> MGSSHHHHHHSQDPENLYFQSMIPQFVIPLTNCLGQSYHFSSQPIPKGEHKKFDSEQSAKAFLDDFVPLRSSRVEELYHLLGQFPPNVPDEELTPELYAPVFAKALVNGSLYVASFPKTKKNATISSEPTPVPKQVKAKSKQNKAHTSSKTQAKNSASAKPLQTGSECHEKAGDPVSLVTGAEILTLNDVELPNGFVWSRTYRSSKASRNQGLGYGWRHAFQFELKEVTDEKHNVTSWEFISDSADEIEFEPVEHGSTSYQVYVGASCHFLNPNIRIVTLSSGDQYRFELVEDIWLLKQVRNGIFSTFQLRYSRNHRLIEVAHNKRPVLECQYDKQGRLVELLNAKTEQVLTTYIYDEQDDLVGATNDLGLTERYEYQDQHLIAKRVRPTGFTHYFEWSGEGSSAKCIRNFGDSGIYDYRFHYEGAKSSYSDSLDNEWTFIHDEQGHLLEKSSPTGRTWQWHYDHLGRKEKAVFPDNSTTQYQYNQQGQLISKLHSSGAQIQYGYDSLGKLVKTVSPDGDLEKAYYNSLGQRVWDIDALGCVTEYEYDKHGQVVKRESEDGKKSRWWWDKQQRLVAHEVDGTLLRYSYGATDLVNGIAYPDGCVAQISYDDYGRRTSIRYFNDEDKVGYSEEYAYDEFSRVAQIQTPEGVTSYQWGALAQQEAVIFPDGSHISYEYDQQRNLTKLVRSDGLAFEFWYDSEGLLSGTVGFDGLHSQFKYDSMGRIIRKDVADRTVLYSYDDAGF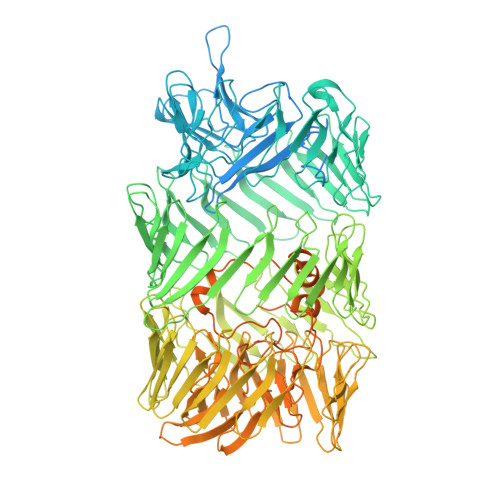LQHIKAGNGKNIVENHFNYTLGGRLTLASNRHQTLQYQYSSFGHLTKRIQGQFEIGEEFNRVGQRVSQTLPDKTSFNFSYDTNGRLSEIRFSDDSLPKIEFQYDVMGRLSVTETESFRESKLYDGVGRLVEQQWSGREKKYIYNAQNRISSILDNTAGATHYQYDTLGYVTKVSEAGSTSTFESDSFGNPALADSKVMSDRIEAYAGVRYKYDQQGNQVKREGDGTVQKRVFDALSQLVEVHGDSSISHYEYDALGRRTKKITQNGITEFLWEGERLLGERTADGFRWYLYQPETYIPLAVLENGSIYLYECDQVGKPERLKDSAGNIVWSASYDVHGFASIDVEEVRNPLRFQGQYFDQETNLHYNLARYYDPKLGRFIQQDPISIAGGINHYQYAVNPIQWIAPTGFLCEEGLKRLQQMLAEYQAQSDVPQEVCDQILEAAKESSVGEDGVRSQVKIRKPNGKNNIRYEYDLDHIDCKKNEITFYRHINYSDGSKRKIQYTVGIEGFVDIYDFVNVQKCDAQVYDTKTSKTVGGRKIINSEFAGKTVTTKGGDVRFDSDGFPDFTPYSKKTVRVIGLTGDMANDVPLAMARAKITKYDKSKYVWHHHQDGKTMMLIPKSVHSVRNGGVAATGGRSVIQHNLLNPNNKLNYSSPEELV> MGKIGIFFGTDSGNAEAIAEKISKAIGNAEVVDVAKASKEQFNSFTKVILVAPTAGAGDLQTDWEDFLGTLEASDFANKTIGLVGLGDQDTYSETFAEGIFHIYEKAKAGKVVGQTST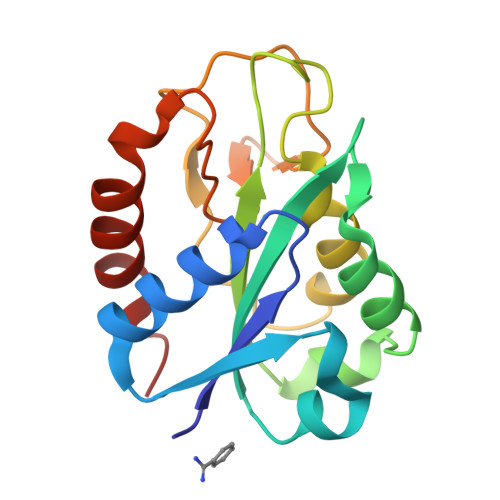DGYHFEASKAVEGGKFVGLVIDEDNQDDLTDERISKWVEQVKGSFA> DLPKFGELLQNVTVPVSREAVLQCVVDNLQTYKIAWLRVDTQTILTIQNHVITKNHRMSITHAEKRAWILRI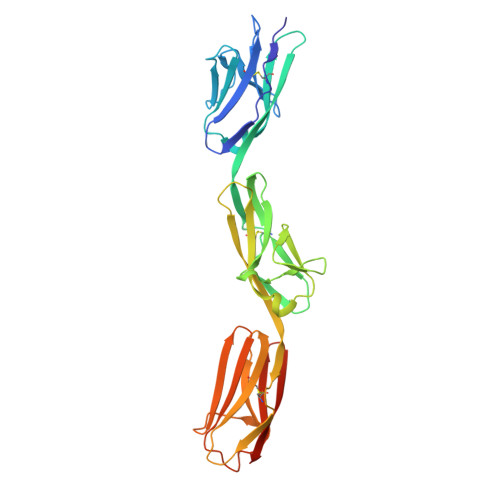RDVKESDKGWYMCQINTDPMKSQVGYLDVVVPPDILDYPTSTDMVIREGSNVTLKCAATGSPTPTITWRREGGELIPLPNGAEAVAYNGSFLTIAKVNRLNMGAYLCIASNGIPPTVSKRVMLIVHFPPMIWIQNQLVGAALTQNITLECQSEAYPKSINYWMKNDTIIVPGERFVPETFESGYKITMRLTIYEVDIQDFGAYRCVAKNSLGDTDGAIKLYHIPHHHHHH> MHHHHHHGAQPARSANDTVVVGSINFTEGIIVANMVAEMIEAHTDLKVVRKLNLGGENVNFEAIKRGGANNGIDIYVEYTGHGLVDILGFPSSTDPEGAYETVKKEYKRKWNIVWLKPLGF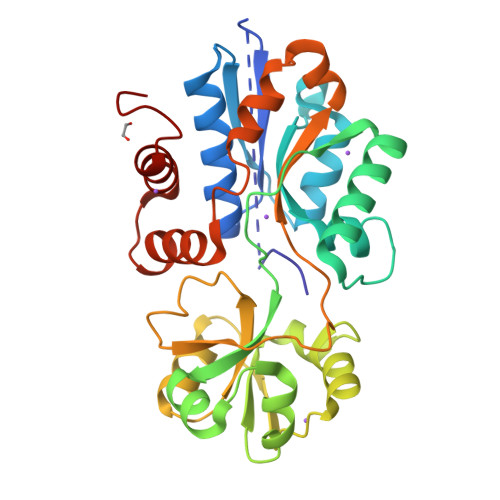NNTYTLTVKDELAKQYNLKTFSDLAKISDKLILGATMFFLEGPDGYPGLQKLYNFKFKHTKSMDMGIRYTAIDNNEVQVIDAWATDGLLVSHKLKILEDDKAFFPPYYAAPIIRQDVLDKHPELKDVLNKLANQISLEEMQKLNYKVDGEGQDPAKVAKEFLKEKGLILQVD>MFQRSIPALITPFTKDNLIDEDSFVDHIEWQISEGSSGLVPAGTTGES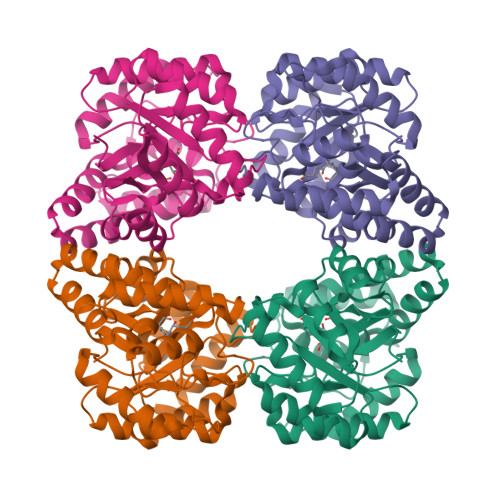STLSYEEHCRVVELCVKTAAGRVPVMAGAGSNNTKESIELAQYAQNTGADALLVVVPYYNKPNKKGLLAHFGSIANAVSLPIYIYNNPSRTVIEMDVDTMAELVKTYSNIVGVKDATGRIELASGQRIACGSDFIQLSGDDSSALGFNVHGGVGCISVTANVAPRICAEFQKAISEGDYRQALEYQDKLFPLHQALFIEPSISSVKYALSRLGRNVSLVVRAPMVSILEKETMFAIDQALDHIGLCAG[6x]AMINOMETHYLCYCLOHEXANE | C7 H16 N 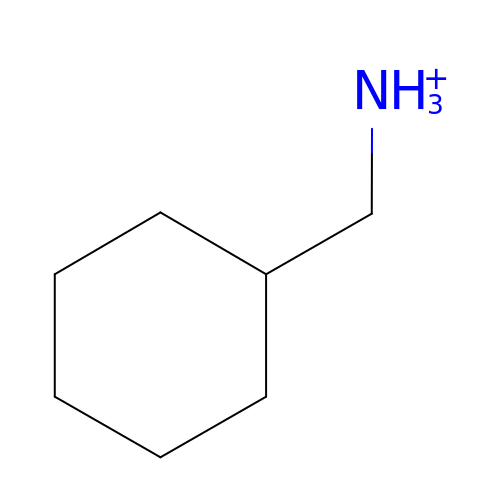| AVKNGPAMCBSNSO-UHFFFAOYSA-O> EKVQAKGMGFGGNRKIGEYQFGKDLPLLEITRDSSVEMCFMENTDVKVVDMGHKYYSNNKPMQFTCKETPDTQSTKTYYT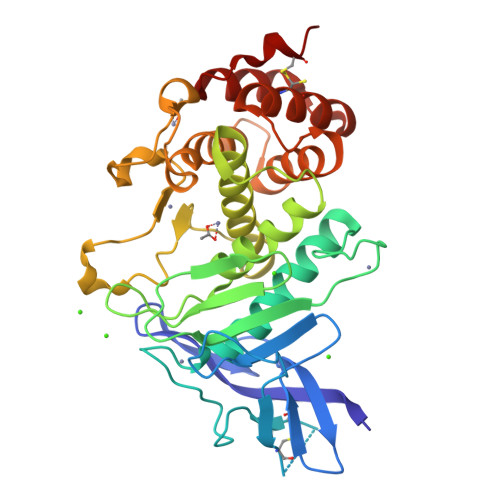GYSADGYDRDNGAASPTNDALYAGYVIKHMYHDWYGVEALTKSDGSPMQLVMRVHYGQGYENAYWDGKQMTFGDGDTMMYPLVSLGVGGHEVSHGFTEQHSGLEYFGQSGGMNESFSDMAAQAAEYYSVGKNSWQIGPEIMKEDSGYDALRYMDKPSRDGMSIDVADDYYGGLDVHYSSGVYNHLFYILANQPNWNLRMAFDVMVKANMDYWTPYSTFDEGGCGMLSAAKDLGYNLDDIKKSLSEVTINYQSCYVD>PRLTRRLTGFLPQEIKSIDTMIPLLSRALWNKHQVKKFNKAEDFQDRFIDHVETTLARSLYNCDDMVAYEAASMSIRDNLVIDWNKTQQKFTTRDPKRVYYLSLEFLMGRALDNALINMKIEDPEDPAASKGKPREMIKGALDELGFKLEDVLDQEPDAGLGNGGLGRLAACFVDSMATEGIPAWGYGLRYEYGIFAQKIIDGYQVETPDYWLNSGNPWEIERNEVQIPVTFYGYVDRPEGGKTTLSASQWIGGERVLAVAYDFPVPGFKTSNVNNLRLWQARPTTEFDLNKFNNGDYKNSVAQQQRAESITAVLYPNDNFAQGKELRLKQQYFWCAASLHDILRRFKKSKRPWTEFPDQVAIQLNDTHPTLAIVELQRVLVDLEKLDWHEAWDIVTKTFAYTNHTVMQEALEKWPRRLFGHLLPRHLEIIYDINWFFLEDVAKKFPKDVDLLSRISIIEENSPERQIRMAFLAIVGSHKVNGVVELHSELIKTTIFKDFIKFYGPSKFVNVTNGITPRRWLKQANPSLAKLISETLNDPTEEYLLDMAKLTQLEKYVEDKEFLKKWNQVKLNNKIRLVDLIKKENDGVDIINREYLDDTLFDMQVKRIHEYKRQQLNVFGIIYRYLAMKNMLKNGASIEEVARKYPRKVSIFGGKSAPGYYMAKLIIKLINCVADIVNNDESIEHLLKVVFVADYNVSKAEIIIPASDLSE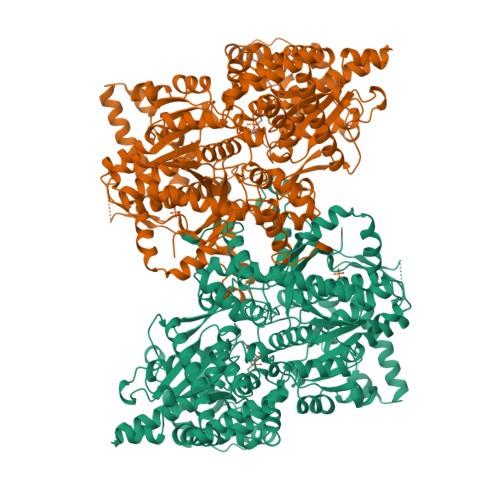HISTAGTEASGTSNMKFVMNGGLIIGTVDGANVEITREIGEDNVFLFGNLSENVEELRYNHQYHPQDLPSSLDSVLSYIESGQFSPENPNEFKPLVDSIKYHGDYYLVSDDFESYLATHELVDQEFHNQRSEWLKKSVLSLANVGFFSSDRCIEEYSDTIWNVEPVT[2x]Endothelin type B receptor (ETBR) plays a crucial role in regulating blood pressure and humoral homeostasis, making it an important therapeutic target for related diseases. ETBR activation by the endogenous peptide hormones endothelin (ET)−1–3 stimulates several signaling pathways, including Gs, Gi/o, Gq/11, G12/13, and β-arrestin. In this study, we present the cryo-EM structure of the ETBR–Gi complex, complemented by MD simulations and functional studies. These investigations reveal an unusual movement of TM7 to the intracellular side during ETBR activation and the essential roles of the diverse NPxxL motif in stabilizing the active conformation of ETBR and organizing the assembly of the binding pocket for the α5 helix of Gi protein.

Furthermore, we performed focused 3D refinement to obtain receptor densities at a resolution of 3.6 Å. Receptor density was assessed in the ETBR–DNGi1 complex after adjusting the alignment center to the receptor. Compared with the ET-1 bound ETBR model in ETBR–DNGi1, the small RMSD values of the Cα atoms and the similar residue conformations in the other two models indicate they are nearly identical (0.391 Å for ETBR–wild-type Gi1 and 0.364 Å for the focused 3D refinement of ETBR). The mode of ET-1 binding in the ETBR–Gi complex closely resembled that of the crystal structure of ET-1-bound ETBR. Y13ET-1 and F14ET-1 in the helical region of ET-1 played a pivotal role in the compact assembly of the N-terminal tail and the extracellular side of TM7, initiating helical rearrangements of ETBR. The C-terminal region of ET-1 (L17ET-1–W21ET-1) fits into the transmembrane orthosteric pocket of the receptor, interacting with many hydrophobic (I1572.60, L2775.42, L3396.51, etc.) and hydrophilic (including K1823.33, K2735.38, R3436.55, D3687.35, etc.) residues. The C-terminal side chain of W21ET-1 directly interacted with W3366.48 in the CWxP motif. Interactions between ET-1 and ETBR, both in the transmembrane region surrounding the C-terminal region of ET-1 and close to the extracellular side, played a role in ETBR activation. These ligand–receptor interactions influenced the helical rearrangement of ETBR through the conserved V1893.40P2855.50F3326.44 motif, resulting in an inward rotation of R1993.50 and Y2935.58, an outward movement of the cytoplasmic side of TM6, and crevice formation on the cytoplasmic side of the receptor to accommodate Gαi. A simultaneous downward displacement (~ 1.5 Å) at the NPxxL motif (N3827.49, P3837.50, and L3867.53 in ETBR instead of Y7.53) was observed in the ET-1–ETBR–Gi complex. N3827.49 extended toward R1993.50, and L3867.53 formed a hydrophobic interaction with I1402.43 to stabilize the helical contacts between TM2 and TM7.

> CSCSSLMDKECVYFCHLDIIW;> PGGGLAPAEVPKGDRTAGSPPRTISPPPCQGPIEIKETFKYINTVVSCLVFVLGIIGNSTLLYIIYKNKCMRNGPNILIASLALGDLLHIVIDIPINVYKLLAEDWPFGAEMCKLVPFIQKASVGITVLSLCALSIDRYRAVASWSRIKGIGVPKWTAVEIVLIWVVSVVLAVPEAIGFDIITMDYKGSYLRICLLHPVQKTAFMQFYKTAKDWWLFSFYFCLPLAITAFFYTLMTCEMLRKKSGMQIALNDHLKQRREVAKTVFCLVLVFALCWLPLHLSRILKLTLYNQNDPNRCELLSFLLVLDYIGINMASLNSCINPIALYLVSKRFKNAFKSALCCWAQS> MTELKNDRYLRALLRQPVDVTPVWMMRQAGRYLPEYKATRAQAGDFMSLCKNAELACEVTLQPLRRYPLDAAILFSDILTVPDAMGLGLYFEAGEGPRFTSPVTCKADVDKLPIPDPEDELGYVMNAVRTIRHELKGEVPLIGFSGSPWTLATYMVEGGSSKAFTVIKKMMYADPQALHALLDKLAKSVTLYLNAQIKAGAQAVMIFDTWGGVLTGRDY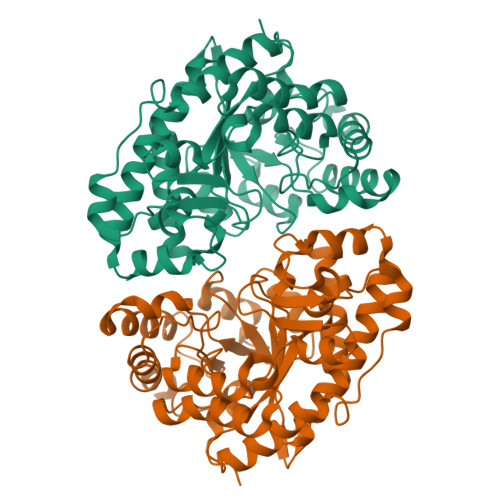QQFSLYYMHKIVDGLLRENDGRRVPVTLFTKGGGQWLEAMAETGCDALGLDWTTDIADARRRVGNKVALQGNMDPSMLYAPPARIEEEVATILAGFGHGEGHVFNLGHGIHQDVPPEHAGVFVEAVHRLSEQYHR> FACKTANGTAIPIGGGSANVYVNLAPVVNVGQNLVVDLSTQIF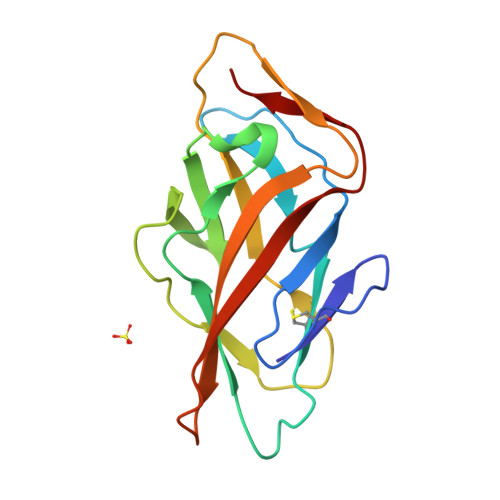CHNDYPETITDYVTLQPGSAYGGVLSNFSGTVKYSGSSYPFPTTSETPRVVYNSRTDKPWPVALYLTPVSSAGGVAIKAGSLIAVLILRQTNNYNSDDFQFVWNIYANNDVVVPTG(1R,3R,7E,17beta)-17-{(1S,2E,5R)-5-hydroxy-1-methyl-6-[(3S,5S,7S)-tricyclo[3.3.1.1~3,7~]dec-1-yl]hex-2-en-1-yl}-2-methylidene-9,10-secoestra-5,7-diene-1,3-diol | C36 H54 O3 | 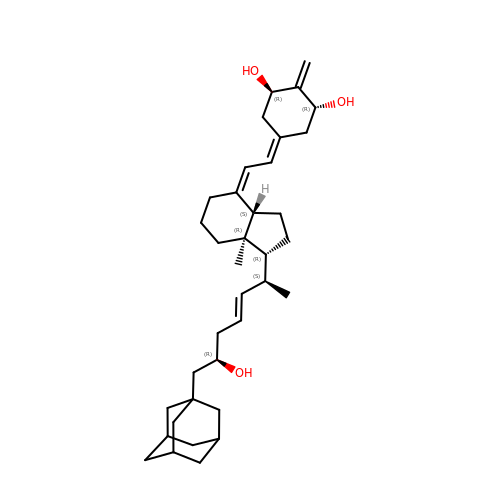GRHLVEDNKGFBSH-QTTWWCOESA-N>SKINVNVENVSGVQGFLFHTDGKESYGYRAFINGVEIGIKDIETVQGFQQIIPSINISKSDVEAIEKAMKK[2x]

One such Spy-specific endolysin, PlyC, has been characterized using biochemical and structural techniques and shown to be a 114 kDa multimeric holoenzyme. These studies demonstrated that PlyC comprises one PlyCA subunit, harboring two distinct catalytic domains that work synergistically to cleave two different bonds in the peptidoglycan, and eight identical PlyCB subunits that form a symmetrical ring for cell wall recognition. Taken together, the data show that the subunit PlyCB mediates translocation of the PlyC holoenzyme across the plasma membrane, where it is subsequently trafficked and quantitatively lyses intracellular Spy. Nonetheless, our results suggest a moonlighting role based on structural motifs within the PlyCB subunit whereby a cationic binding groove is a central determinant of interaction with plasma membranes and subsequent internalization.

To explore the roles of cationic residues in PlyC, we mutated the exposed Arg and Lys residues on PlyCB to Glu in order to independently determine the role of each mutation in Spy binding and lysis, as well as PlyC cellular uptake. Fluorescence microscopy showed a lack of binding of the PlyCBR66E mutant to Spy while PlyCBK23E and PlyCBK59E, as well as a charge-conserving PlyCBR66K mutant bound comparably to WT (left). Moreover, the PlyCBK23E, PlyCBK59E, and PlyCBR66E mutants, but not PlyCBR66K, lost the ability to enter A549 epithelial cells (right). Thus, K23 of PlyCB is not involved in Spy binding but is involved in epithelial cell internalization, whereas K59 and, to a greater extent, R66 are involved in both Spy binding and internalization. PlyCBK59E and PlyCBR66E that lack the ability to internalize in epithelial cells also lost the ability to bind PI and showed diminished binding to PA and PS. To confirm the PS specificity of PlyCB interaction with the membrane, we also measured the membrane affinity of PlyCBR66E. As expected, this mutant binds poorly to PS, comparable with WT PlyCB to PI-containing membranes (compare Figure 5d and Figure 5a). The orange sphere shows the location of a putative phosphate site observed in WT PlyCB in the presence of phosphate or phosphate-bearing ligands. This site holds a water molecule in the WT structure, but an empty site was observed in PlyCBR66E, apparently disrupted by the mutation. The H-bond interaction between R66 and E36 is maintained in the mutant, suggesting that the observed side-chain conformations represent a stable configuration.> AQPDIKFASKEYGVTIGESRIIYPLDAAGVMVSVKNTQDYPVLIQSRIYDENKEKESEDPFVVTPPLFRLDAKQQNSLRIAQAGGVFPRDKESLKWLCVKGIPPKDEDIWVDDATNKQKFNPDKDKDTNDVGVFVQFAINNCIKLLVRPNELKGTPIQFAENLSWKVDGGKLIAENPSPFYMNIGELTFGGKSIPSHYIPPKSTWAFDLPKGLAGARNVSWRIINDQGGLDRLYS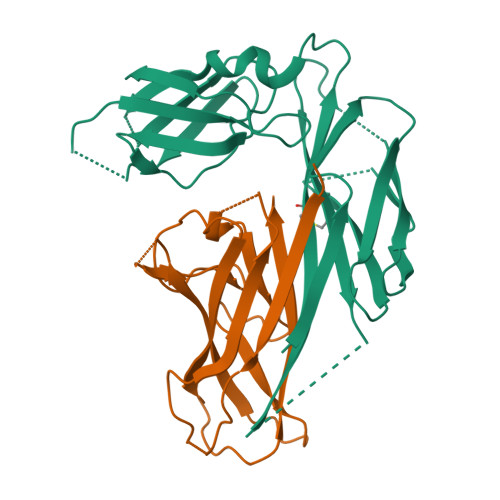KNVTL;> ADLTASTTATATLVEPARITLTYKEGAPITIMDNGNIDTELLVGTLTLGGYKTGTTSTSVNFTDAAGDPMYLTFTSQDGNNHQFTTKVIGKDSRDFDISPKVNGENLVGDDVVLATGSQDFFVRSIGSKGGKLAAGKYTDAVTVTVSNQ>GSHMRVQVSGLSDETTWHTLKDHLRQAGEVTFCKVFSGGRAVVEFVTPEDAARAITELQASELEGATLFLR[9x]

Kinetoplastid RNA (kRNA) editing takes place in the mitochondria of kinetoplastid protists and creates translatable mRNAs by uridine insertion/deletion. TbRGG2 is a 330 residue protein and contains two main domains, an N-terminal glycine (Gly)-rich region composed of GWG and RG repeats and a C-terminal RNA recognition motif (RRM). Unlike these editing accessory proteins, the T. bruceiRGG2 (TbRGG2) protein is required for editing all nine pan-edited mRNAs. TbRGG2 binds RNA and modulates RNA structure and these functionalities have been shown to be to be essential for its role in kRNA editing.

To determine how the TbRGG2 RRM domain binds RNA, we obtained the structure of the domain bound to a poly-uridine (U4) RNA. The structure was solved by molecular replacement and refined to final Rwork/Rfree values of 18.1%/22.9% to 1.95 Å resolution. Comparison of the RNA-bound RRM domains with that of the apo RRM structure shows no significant structural changes take place upon U4 RNA binding. The TbRGG2-RNA structure has a complex asymmetric unit. However, four similar TbRGG2 RNA complexes were revealed. In each of these complexes two RRMs combine to simultaneously contact one RNA using a unique binding mode distinct from that observed in other RRM–RNA complexes. In the TbRGG2-RNA complex, key RNA base stacking interactions are provided by Phe230 from β-strand 2 and Trp215 from the N-terminus of α-helix 1, from two RRM subunits. In this novel RRM-RNA interaction, binding by the two RRMs splays apart the U4 substrate, suggesting a mechanism by which the protein may mediate melting or stabilization of single stranded RNA U stretches. In the TbRGG2 RRM-U4 structure, the uridine O2 and N3 atoms are read by the backbone amide nitrogen and carbonyl oxygen of RRM residue Cys231. In addition to the RNA contacts from the Cys231 backbone and the side chains of Phe230 and Trp215, several basic residues either make contacts to the RNA phosphate backbone (Lys219) or are positioned to provide electrostatic contacts to the RNA, such as Lys230.> HHHHHHGP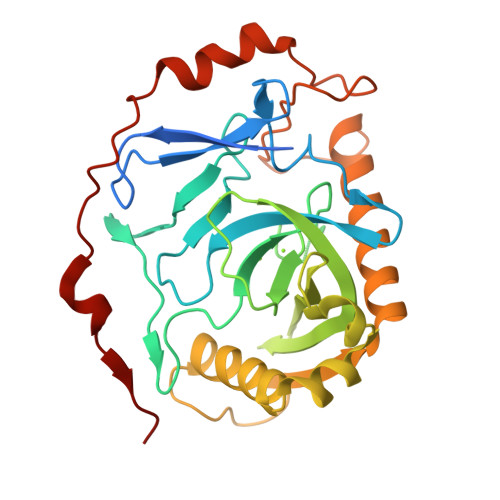NTEFALSLLREFMSGFSTEERAAPFSLEYRVFLKNEKGQYISPFHDIPIYADKDVFHMVVEVPRWSNAKMEIATKDPLNPIKQDVKKGKLRYVANLFPYKGYIWNYGAIPQTWEDPGHNDKHTGCCGDNDPIDVCEIGSKVCARGEIIGVKVLGILAMIDEGETDWKVIAINVDDPDAANYNDINDVKRLKPGYLEATVDWFRRYKVPDGKPENEFAFNAEFKDKDFAIDIIKSTHDHWKALVTKKTNGKGISCMNTTLSESPFKCDPDAARAIVDALPPPCESACTVPTDVDKWFHHQKN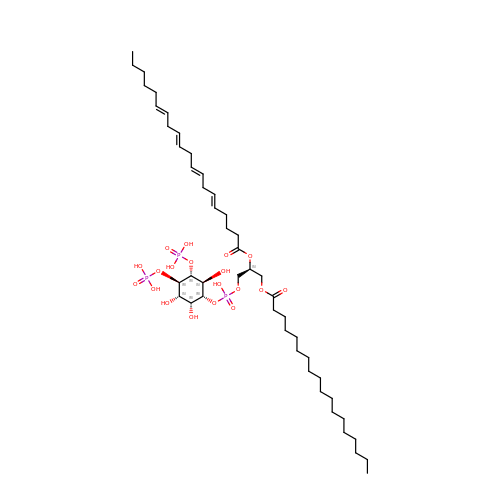(2S)-1-{[(R)-hydroxy{[(1R,2R,3S,4R,5R,6S)-2,3,6-trihydroxy-4,5-bis(phosphonooxy)cyclohexyl]oxy}phosphoryl]oxy}-3-(octadecanoyloxy)propan-2-yl icosa-5,8,11,14-tetraenoate | C47 H85 O19 P3 | CNWINRVXAYPOMW-AUBJPSKUSA-N> XEWEALEKKLAACESK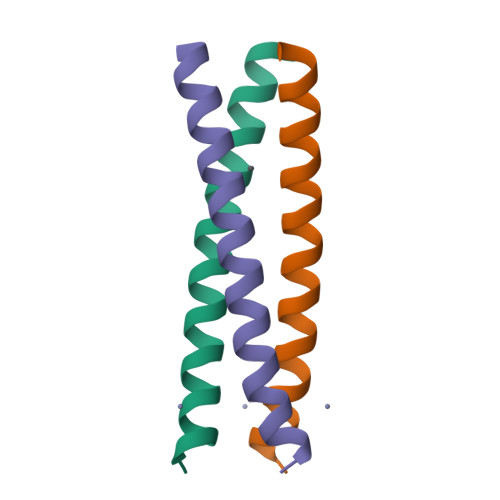AQALEKKLQALEKKLEALEHGX>[8x]MADVPAGVTLAEKQTLVRNNGSEVQSLDPHKIEGVPESNISRDLFEGLLVSDLDGHPAPGVAESWDNKDAKVWTFHLRKDAKWSDGTPVTAQDFVYSWQRSVDPNTASPYASYLQYGHIAGIDEILEGKKPITDLGVKAIDDHTLEVTLSEPVPYFYKLLVHPSTSPVPKAAIEKFGEKWTQPGNIVTNGAYTLKDWVVNERIVLERSPTYWNNAKTVINQVTYLPIASEVTDVNRYRSGEIDMTNNSMPIELFQKLKKEIPDEVHVDPYLCTYYYEINNQKPPFNDVRVRT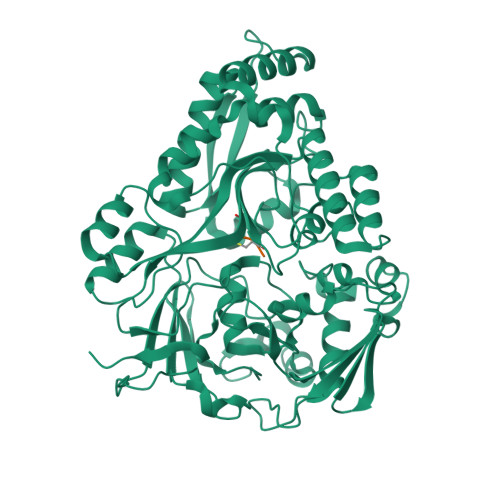ALKLGMDRDIIVNKVKAQGNMPAYGYTPPYTDGAKLTQPEWFGWSQEKRNEEAKKLLAEAGYTADKPLTINLLYNTSDLHKKLAIAASSLWKKNIGVNVKLVNQEWKTFLDTRHQGTFDVARAGWCADYNEPTSFLNTMLSNSSMNTAHYKSPAFDSIMAETLKVTDEAQRTALYTKAEQQLDKDSAIVPVYYYVNARLVKPWVGGYTGKDPLDNTYTRNMYIVKHHHHHHH In this study, we biochemically characterized one such protein, UMAG_00027, that is highly expressed during plant infection. We show that UMAG_00027 is a secreted protein with a lectin-like fold and therefore term it Llp1 (lectin-like-protein 1). Llp1 decorated the fungal cell wall of cells grown in axenic culture or proliferating in planta, which is in agreement with its potential sugar-binding ability. CRISPR/Cas9-mediated deletion of llp1 reveals that the gene is not essential for fungal virulence.

The protein fused to a C-terminal hexa-histidine tag, was expressed in Escherichia coli SHuffle T7 cells and enriched via a two-step purification protocol combining nickel ion affinity chromatography and size exclusion chromatography (SEC). Diffraction data were collected at 2.01 Å resolution at the EMBL beamline P14 (Deutsches Elektronen-Synchrotron; DESY) under cryogenic conditions. Due to the absence of known structures suitable for molecular replacement, we employed isomorphous replacement using single-wavelength anomalous dispersion data obtained from selenomethionine incorporation. Amino acid residues 23–241 of Llp1 could be unambiguously assigned to the electron-density map and represent almost all the residues of the protein construct employed in this study (Note: N-terminal 22 residues comprising the signal peptide were not present in the Llp1 expression construct). The secondary structure elements are connected by several loops, which contain four small helices. In total, the molecule has three exposed disulfide bonds probably conserved among orthologs. Overall, this results in a compact and stable molecular fold. Taken together, our structural analysis shows that Llp1 has a high structural similarity to members of the carbohydrate-binding concanavalin A-like (ConA) lectin/glucanase family. Despite extensive efforts with microscale thermophoresis (MST), we could not detect the specific binding of Llp1 to a variety of sugars such as chitobiose, chitotetraose, N-acetylglucosamine, rhamnose, cellobiose, galactose, arabinose, mannose, maltotriose, and glucose.

> MGPLQCHMQAFNANIISVDAYSANDLSDKHAPLGASGYFADVTLTGKYHQDVFDARHWLTMRHSGTDCRNVKGTDSKVCNIDYVENQPGNSCAQVTQRSHLLGWSSGKALDISATAPNAPVHFRASLAPSLQTWWTGLPNTCAVQRYNAPHNPYKIVTLTASGMHTWTKLVIMLDAPEPSFFKSWSCEYNDSLSPVVGNIQVSEDGKTYTLTNVKYQPILYSANEENKSLEHHHHHH> MKWIYKFDVLYQSRNPRYRNYEIIRTNVQEVLAEIVSPSTKNPNSENPAVKKRFRGIKNVVSRIISNDKKCRYDLIYNKYLSSSDTRKLKTMIDYSTKFNRVVEVVLIIMGKLLP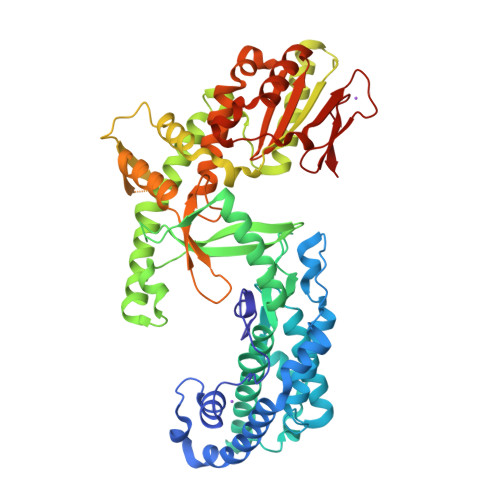LDAWGGTENKKVIQDRIVDFLRLGANERLHLDDVLSGIKLSKFKWLGVGNNISSQQDFQIRKRLLEGYINWVFISLVKNIVRAFWYVTESSNMDRSKLFYFTHSIWNELSSNWITKYAKGNLVQVVSPESKGQFTNGKIKLIPKRGGFRVICVPLKQSLYSFNNKRNFALKQKEKWDYIFYQKYTLSPVRQVLQLKLNALRKSDMGHRSSVNSTNEVADRILTFRNDLLKKNKTLPVLYMIKFDMKECYDRLNQNALKESIAGIFKEDNENTTYHVREYGTLDEFLKLKRVRTLIETEVQNFNIIMNSKDEAEAGSRSYGTKVDKVKTLSISKNKIIEVCHSQIEDATCLVKNKEGQYDLFKRKQGVFQGFSLSGIFCDILYSTMVSKEFKFLWEATEDNLLLRLVDDFIFITSNKDTLKKVKDKISSNELQKYGAFVNHEKTVEINGEAGSSNKMTFVGLDINCLTLDVKKDSVD>[2x]MTMEQFLTSLDMIRSGCAPKFKLKTEDLDRLRVGDFNFPPSQDLMCYTKCVALMAGTVNKKGEFNAPKALAQLPHLVPPEMMEMSRKSVEACRDTHKQF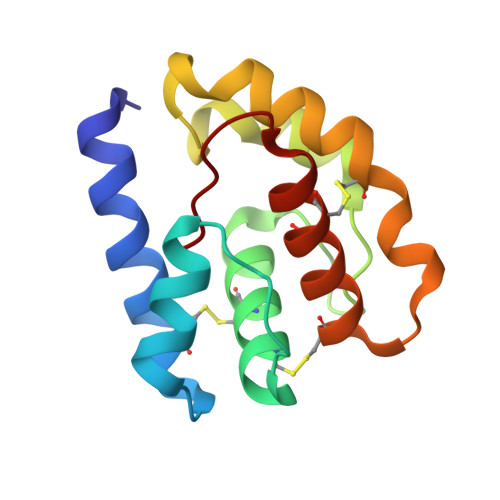KESCERVYQTAKCFSENADGQFMWP>MSFVEDYLTKLQERPTIIENPNILKGSKIFNAIYRVDDFVYIHIQSIKSEDGYNQYNVIEPPRPTHDEMEEIEEKFALSIGDKEPPEDTKEKEKLIRSILDKILLRMRLSVPKEYVIYHFIRDKLYTGSLEPLIRDPYIEDISIPGLGHVYIVHKVFGPMRTSIKFENYEELDNLIVSLSEKSY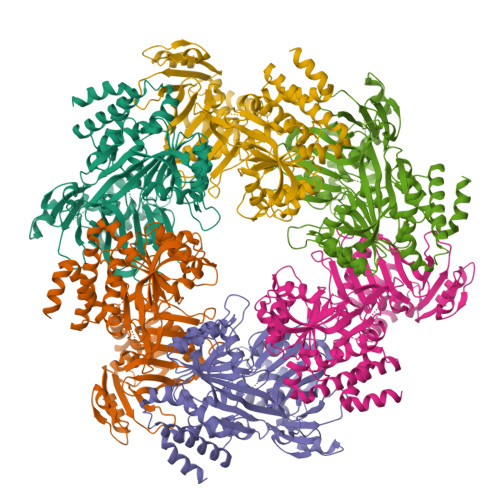RPVSHNRPVVDASLPDGSRVNFVYGVDISRRGSNLTVRKFSRVPTSITQLIMFGTLSSMMAAYIWTMLDEGMNLFVCGETASGKTTTLNAITAFIPPNLKIVTIEDTPELTVPHSNWVAEVTRETGGEGTIKLFDLLKAALRQRPNYILVGEIRDKEGNVAFQAMQTGHSVMATFHAANITTLIQRLTGYPIEVPKSYINNLNIALFQTALYDKKGNLIRRVVEVDEIIDIDPVTNDVVYIPAFTYDSVQDKMLFAGKGSSYLIENKIAVKRGIDRRNIGLLYDELQMRSRFLNLLVEKKIFNYYDVWDYILRARQMGLEEAIKYVSNI[4x]>FACKTANGTAIPIGGGSANVYVNLAPAVNVGQNLVVDLSTQIFCHNDYPETITDYVTLQRGSAYGGVLSSFSGTVKYNGSSYPFPTTSETPRVVYNSRTDKPWPVALYLTPVSSAGGVAIKAGSLIAVLILRQTNNYNSDDFQFVWNIYANNDVVVPTGGCDVSARDVTVTLPDYPGSVPIPLTVYCAKSQNLGYYLSGTTADAGNSIFTNTASFSPAQGVGVQLTRNGTIIPANNTVSLGAVGTSAVSLGLTANYARTGGQVTAGNVQSIIGVTFVYQ[2x];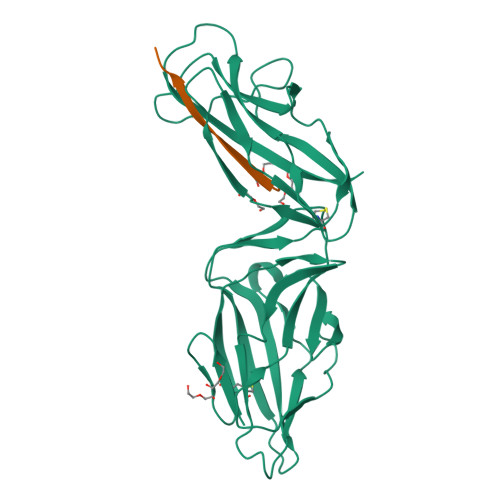>ADVTITVNGKVVAK[2x]PsEst3, a psychrophilic esterase obtained from Paenibacillus sp. R4, which was isolated from the permafrost of Alaska, exhibits relatively high activity at low temperatures. Here, crystal structures of PsEst3 complexed with various ligands were generated and studied at atomic resolution, and biochemical studies were performed to analyze the structure–function relationship of PsEst3. The residues located in the active site, including the catalytic triad (Ser128, Asp199 and His227), were strictly conserved.

Four structures were obtained: a sulfate-bound form, the wild type bound to PMSF, a malonate-bound form of the S128A mutant and an apo form of the S128A mutant. The S128A and S128C variants were prepared to investigate whether PsEst3 exhibits the same mechanism as that of dienelactone hydrolase or a classical esterase. Mutational analysis revealed that the activities of both variants were <10% that of the wild type [Fig. 6(c)]. Structural superposition of the sulfate-bound structure and the malonate-bound structure of the S128A mutant with the apo structure of the S128A mutant revealed r.m.s.d.s of 0.4 and 0.3 Å, respectively, indicating that the overall conformational changes caused by the ligands were not critical.

> MGNAVVVKKDFRIDLENELFIRGEVTLVEDQIKKPVLVISHGFRGYKDWGFWPYVAAWFAERGFYVVHFDFSRVGALNSGADEASVQKLSTVSRELSDLDAILSNLREHRLPLAEQAETERISLLGHARAGGSNIIFAAEHSYIGSVIAWNGGPPPKAAAGNPNPFINDDVEHNKQRFDTARLLASLTAPVLIIQGGKDREALLEGQQLLKEAAPNQTYISIPDADHSFGGEHPFHHTTPYLEEALEVTHSFITKHYLEHHHHHH>SETSRTAFGGRRAVPPNNSNAAEDDLPTVELQGVNLRGVNLQEFLNVTSVHLFKERWDTNKVDHHTDKYENNKLIVRRGQSFYVQIDFSRPYDPRRDLFRVEYVIGRYPQENKGTYIPVPIVSELQSGKWGAKIVMREDRSVRLSIQSSPKCIVGKFRMYVAVWTPYGVLRTSRNPETDTYILFNPWCEDDAVYLDNEKEREEYVLNDIGVIFYGEVNDIKTRSWSYGQFEDGILDTCLYVMDRAQMDLSGRGNPIKVSRVGSAMVNAKDDEGVLVGSFDNIYAYGVPPSAWTGSVDILLEYRSSENPVRYGQCWVFAGVFNTFLRCLGIPARIVTNYFSAHDNDANLQMDIFLEEDGNVNSKLTKDSVWNYHCWNEAWMTRPDLPVGFGGWQAVDSTPQENSDGMYRCGPASVQAIKHGHVCFQFDAPFVFAEVNSDLIYITAKKDGTHVVENVDATHIGKLIVTKQIGGDGMMDITDTYKFQEGQEEERLALETALMYGAKKPLNTSRSMKSRSNVDMDFEVENAVLGKDFKLSITFRNNSHNRYTITAYLSANITFYTGVPKAEFKKETFDVTLEPLSFKKEAVLIQAGEYMGQLLEQASLHFFVTARINETRDVLAKQKSTVLT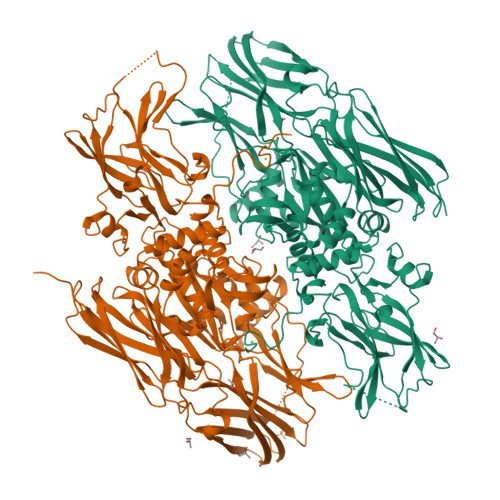IPEIIIKVRGTQVVGSDMTVTVQFTNPLKETLRNVWVHLDGPGVTRPMKKMFREIRPNSTVQWEEVCRPWVSGHRKLIASMSSDSLRHVYGELDVQIQRRPSM[2x]Briefly, as implied from its name, the CU system transports its protein cargo, known as pilus subunits, across periplasm and outer membrane in a relay manner mediated by two functionally conserved proteins known as a periplasmic chaperone and an outer membrane usher. In this study, we report the crystal structure of P. aeruginosa CupB2. Similar to other CU chaperones, the CupB2 structure reveals a classical boomerang-like fold consisting of two immunoglobulin (Ig)-like domains. With the structural and biochemical data presented here, it is now clear that CupB2 is an FGS-type chaperone with two functionally different Ig domains.

The unit cell contains two CupB2 polypeptide chains per asymmetric unit, which were refined independently. Other disordered regions include residues 125–133, 166–173, 217–222 and 248 in chain A and residues 123–136, 165–172, 217–224 and 247–248 in chain B. The structures of the CupB2 chains in the asymmetric unit are very similar with a root mean square deviation (RMSD) in Cα position of 0.3 Å. Size exclusion chromatography of CupB2 is in agreement with a monomeric protein in solution. Hence, unlike the PapD and Caf1M chaperones, there is no self-capping relationship among CupB2 molecules. The N- and C-terminal domains are connected by a kinked linker, residues 145–152. The relative orientation of these two domains are stabilized mainly by polar interactions involving the side-chains of Glu111, Arg145, Tyr183 and the main-chains of Arg110, Pro146, Lue149, Lys150, Ser151, Pro182 and Tyr184. Interestingly, these residues are all located underneath two invariant positively charged residues, Arg36 and Lys141 lying in the cleft formed by the N- and C-terminal domains. Arg36 and Lys141 are well-conserved residues among PapD-like chaperones, where they are involved in the first point of contact with the unfolded subunits exiting the Sec translocon by capturing the emerging C-terminal carboxylate of the subunit's chain. As shown in Figure 3 where CupB2 is superimposed with the structure of the PapD:PapH complex, Arg36 and Lys141, together with the F1–G1 loop, are all in immediate contact with the pilus subunit. Only the biotinylated CupB1 peptide, but not the CupB6 peptide, can pull down the CupB2 chaperone. Consistent with the limited trypsin digestion described above, the CupB1 peptide showed no binding toward the CupB2(R36A) mutant, strongly implying that CupB2 is indeed the periplasmic chaperone for CupB1.

>MAPLMHRFHSFVAASAVAIALCVGTAHAGLIAQGTRVVFPASEREVTLRVSNTSGTPVLAQAWIDDGRQDVPPEELQVPFSVTPAVTRVEPNGGAVLRIAYLKAPLPTDRESLFWLNILEVPPRDEDENNALQFSFRSRFKLFFRPSQLKSVDSAAGKLQWKFLESGGAGKKTVVQVNNPTPYYVSFASVELIVDGRVMSVGKGMVAPFSTKEFDWQGNPKNMEAASVRYEVINDYGGRNTHDRALGKRGSHHHHHH[2x]>[4x]MGSSHHHHHHSSGLVPRGSTKNYYDRSVSPVEYAYFDQSQNMRAINWNKIVDEKDLEVWNRVTQNFWLPENIPVSNDLPSWNELDDDWQQLITRTFTGLTLLDTVQSSIGDVAQIKNSLTEQEQVIYANFAFMVGVHARSYGTIFSTLCTSEQIEEAHEWVVDNEALQARPKALIPFYTADDPLKSKIAAALMPGFLLYGGFYLPFYLSARGKLPNTSDIIRLILRDKVIHNFYSGYK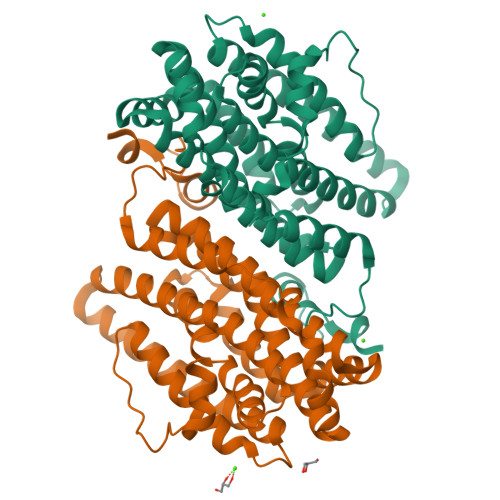YQLKVAKLSPEKQAEMKQFVFDLLDKMIGLEKTYLHQLYDGFGLADEAIRFSLYNAGKFLQNLGYESPFTKEETRIAPEVFAQLSARADENHDFFSGSGSSYIIGTSEETLDEDWDF>[8x]MTENSITAANVEELIAKNIAERFADDHEVLGLSQHFRREGYVKLPGLVSPEVFDAVAAETHQLIDTHQKRIDIRLKETGDSPRYMSTVGQKAIATDGSLIPAVYESTALKGFLSRLAKEEVMGC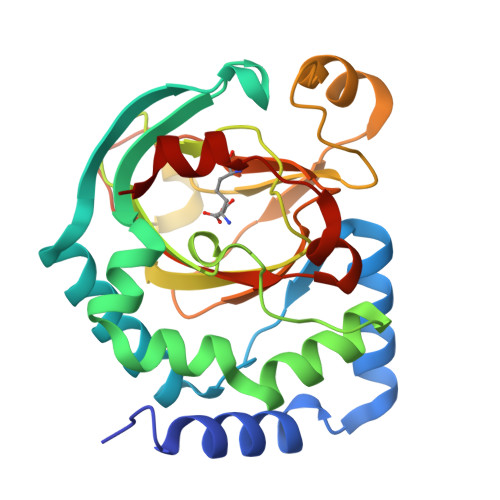PWDEEKYIITRQHQKGDTHGWHWGDFSFTVIWLIEAPSLEYGGMLQCIPHTDWNKDDPRVEDYLQKHPIRSYGHAKGDLYLLRSDTTLHRTVPLNADRTRIILNTCWASRADQQKATTHETMNAMFD>[2x]MKSYEIALIGNPNVGKSTIFNALTGENVYIGNWPGVTVEKKEGEFEYNGEKFKVVDLPGVYSLTANSIDEIIARDYIINEKPD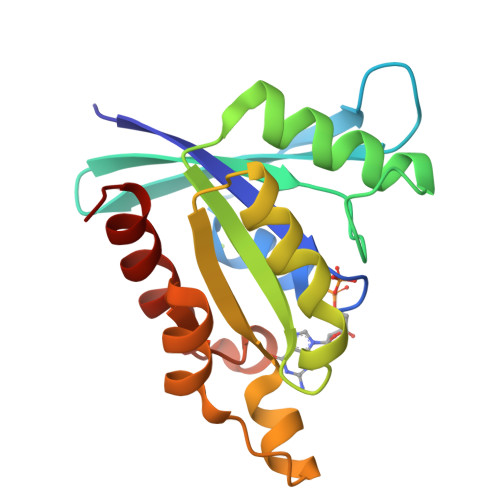LVVNIVDATALERNLYLTLQLMEMGANLLLALNKMDLAKSLGIEIDVDKLEKILGVKVVPLSAAKKMGIEELKKAISIAVKDL> 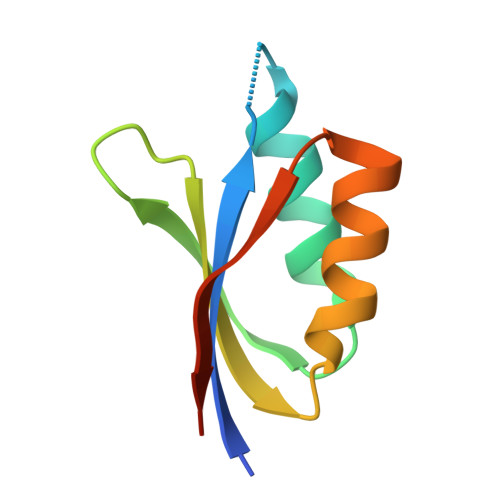GPGLKQKIVIKVAMEGNNCRSKAMALVASTGGVDSVALVGDLRDKIEVVGYGIDPIKLISALRKKVGDAELLQVEQAKED>MVLYFIGLGLYDERDITVKGLEIAKKCDYVFAEFYTSLMAGTTLGRIQKLIGKEIRVLSREDVELNFENIVLPLAKENDVAFLTPGDPLVATTHAELRIRAKRAGVESYVIHAPSIYSAVGITGLHIYKFGKSATVAYPEGNWFPTSYYDVIKENAERGLHTLMFLDIKAEKRMYMTANEAMELLLKV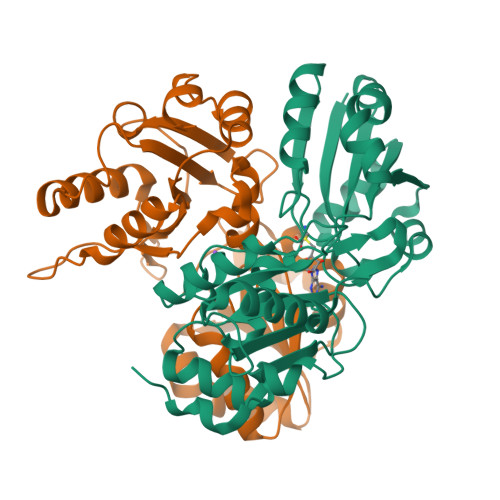EDMKKGGVFTDDTLVVVLARAGSLNPTIRAGYVKDLIREDFGDPPHILIVPGKLHIVEAEYLVEIAGAPREILRVNV[2x]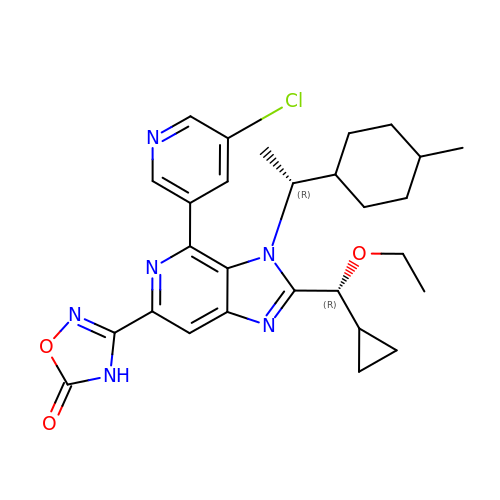3-[4-(5-chloropyridin-3-yl)-2-[(R)-cyclopropyl(ethoxy)methyl]-3-{(1R)-1-[(1r,4R)-4-methylcyclohexyl]ethyl}-3H-imidazo[4,5-c]pyridin-6-yl]-1,2,4-oxadiazol-5(4H)-one | C28 H33 Cl N6 O3 | PJGMHURMTNPVFZ-TYPDQXGPSA-N> DKPFNLRSRDPIYSNNYGKLYEITPEKNSQLRDLDILLNCLQMNEGALFVPHYNS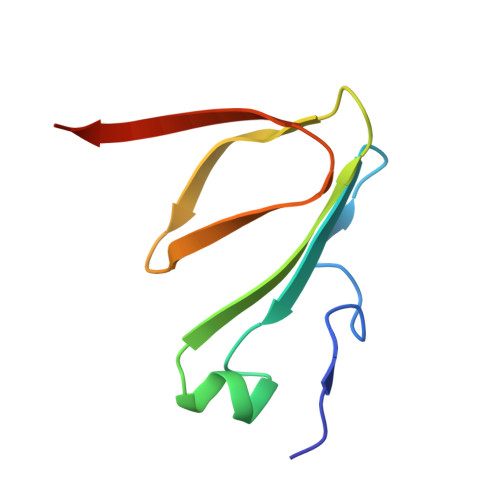RATVILVANEGRAEVELVGLEQQQ> MRLPDPYTNPEYPGLGFESVNLVDNDPMIRDELPNGKV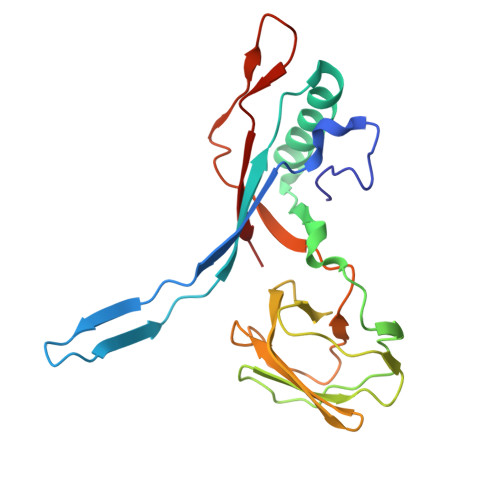KEVKISAQYWGINISYPELFPDEYAFLDSRLLEYKRTGDYLDVLLPQYEAFRVRGDTKSVTIPAGQKGSQIILNTNGTLTGQPKAGDLFKLSTHPKVYKITNFSSSGNVWNISLYPDLFITTTGSEKPVFNGILFRTKLMNGDSFGSTLNNNGTYSGISLSLRESL>[84x]MSGFGGGSSGAGSLTQLLATGSMDAALTQNATRTFWKSSYQKHSLFALESINQPFTTQVQFGAESHITVNRQGDLLSWMYLKIVLPGLKVQNQADTVQPTQQSFASLDNDVAAQADVSHVLPYIEGAYTEASLNTKEQLIAEAKNSYEAAKYNAAPLPVAAQMQSTEMPDFDYAYWTEAIGFHLIKRAEFKVGGATIDTIWSELLFAMEELMGRAGRRLTETIGRTLRRPTELMKASRQEQILYVPLPWYFTKHPSLAFPLVAATYHNIQLWVQWAQLNSCIIKSRSNLVVLHAERNVPISDDHLRASLECTYVHLEAAERDALTANAGTQLIVQHQAHLQQVSSNNVTARLNFNFPVLEFYYFLRRKANKDAGDHFNFSGIGGRDPVVSAELLFNNTARVTQKP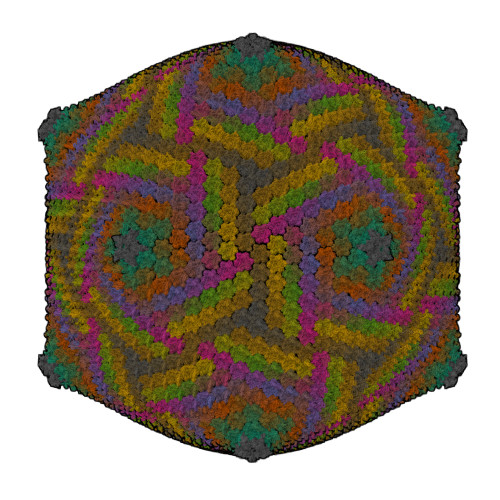AVWWRAVQALQFHSSAPLTNIYSYSFSLSPEDPITPSGSANFSRLDSVELALTLQDDFGAAHDANSELFVFARSYNILKFTNGLAGLLYSN;> MPSIAFSGISTKPGELEFHVPSVLSKHNRAGLLKSIDFPYSQRTIESSWNKLHYMESIRITPESRSVSVLLTDKESGDRVEMLAMVPLTTNKIIEISTATTDGTIILVTEEPHGFFAPGCFGKEVRNVISSYKSIFPHGTPPFILIHGSNGSVQVDPALFEYNDEYSVKIKYTAIRTEFKLFGKGDHGWMVTPEFPTISMLCQVITNAMNSAIIFNHDDPAARTRMYPGTCSNTHVIESVSGDSLAKALLGYDGVYAGWEEITIPAGMYCYGELDLSKMIAAKMNRWHIDRESSIIFRGVSGYTWNVTLPSGNYGTPEKLAHCIQHMMNMTAKNRKNPYCVRFTLNEGSSHRGKFVFVAAEPFDLLFGDDESIDPSILGFEPVDHIGRNSYMSENDLGAPLMKPNCNVYDVDEIPGTHQIRIGRRTRLAVDGKIRGYSGGTLRLNTVNRTTGAPKCHGMNKGDVVTLTTVMPAPDGATGTKREGFTFRAKNKIMGVVVADENENPDASSLHVSVPSMSWTLGIGSYITIDSQAAPISVALFDPGKNQFFRDSIGASRLGFSNGVSTGQHGVVVSQCAVNLEPRTVDVSFIEGSMTSASTEMYNQNGKSLITQVPSDRSSGPVPQGMVRFNNALQQFKLEFTNPDGSPYHFNHASLSLLMEFDD>[4x]RENLYFQGMTEVNLNI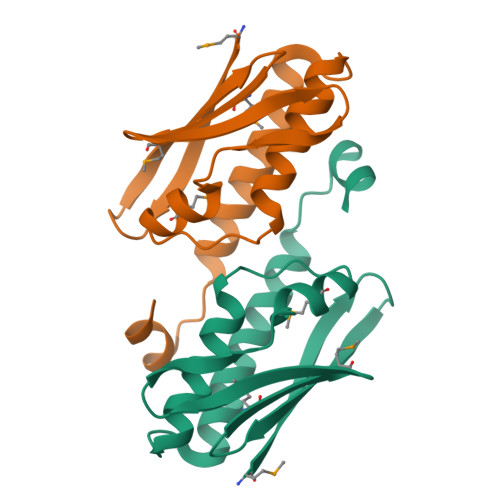YSPRWGRHETYIVELHKDYMEISMGAVTIKATYSENQDPEWSEETLQDIMNNDSVYPPEITQNLFQHAWLEWRKGALDNDEVTRELELVAQWVNKVTEAKPNSDFWRKYF> RRR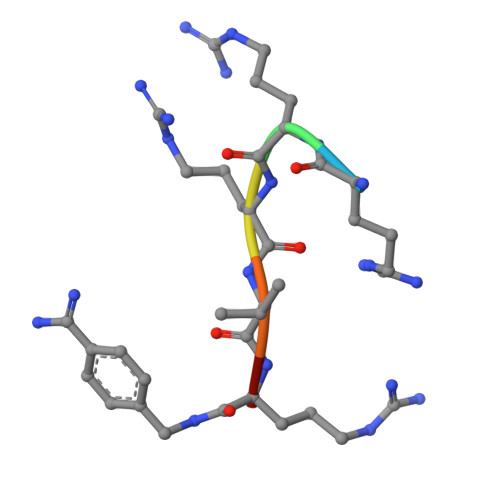VRX>MSTVIKGGTIVTADLTYKADVKVEGGRIVEIGPNLSGAETLDATGCYVMPGGIDPHTHLEMPFMGTYSSDDFESGTRAALAGGTTMVVDFALPSPGQSLLEALTMWDNKSTRANCDYSFHMAITWWGEQVFNEMETIVKDKGINTFKHFMAYKGALMVDDDEMFSSFQRCAALGALPLVHAENGDVVAQLQAKLLAEGNSGPEAHAYSRPAEVEGEAANRAIMIADMAGCPVYIVHTSCEQAHEAIRRARAKGMRVFGEPLIQHLTLDETEYFDKDWDHAARRVMSPPFRNKLHQDSLWAGLASGSLQVVATDHCAFTTEQKRFGVGDFTRIPNGTGGLEDRMPMLWTYGVATGRITMNEFVAVTSTNIAKILNIYPKKGAILVGADADLVVWDPKRSKTISAKTQQSAIDYNVFEGKTVTGLPRFTLTRGVVSIEEGTVKTQEGHGEFVRRDPFPAV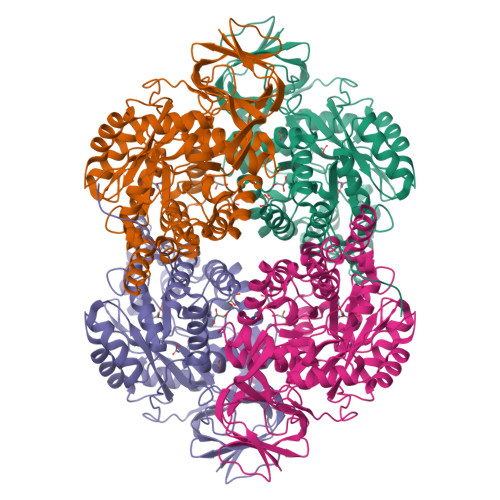STALSTWKEVTAPRAVQRSGIPASGVHHHHHH[2x]In the case of Sqt1, we were able to decipher the mode of L10-N peptide binding by X-ray crystallography. These structural analyses showed that the C-terminal domain of Sqt1, which is preceded by a non-essential N-terminal extension of ∼50 amino acids, folds into an eight-bladed WD-repeat β-propeller. Moreover, the binding mode of the N-terminal residues of Rpl10 (L10-N) by the eight-bladed WD-repeat β-propeller of Sqt1, as revealed by X-ray crystallography, allows establishing a refined model for the final pre-60S maturation events that lead to the stable incorporation of Rpl10 and the release of Nmd3. Taken together, we propose that Sqt1 may protect Rpl10 from aggregation before and/or promote its incorporation into almost mature pre-60S subunits in the cytoplasm. We conclude that the β-propeller domains of Sqt1 and Rrb1, which harbour the essential function of these proteins, recognize the very N-terminal residues of Rpl10 and Rpl3.

To this end, we also performed in vitro binding assays with the orthologous proteins from the thermophilic, filamentous ascomycete Chaetomium thermophilum (ct), whose proteins often exhibit improved biochemical properties. Both ctSqt1 and ctSqt1.52C (deletion of amino acids 2–51), which fully complement the absence of Sqt1 in vivo, could be efficiently co-purified with ctRpl10 or its N-terminal 20 residues. As a first step towards the elucidation of the recognition mode of the N-terminal residues of Rpl10 by the predicted β-propeller domain of Sqt1 at the atomic level, we independently determined the crystal structure of ctSqt1 at 1.94 Å by molecular replacement and of ctSqt1.52C, lacking the dispensable N-terminal extension, at 1.5 Å resolution by single-anomalous dispersion (SAD) followed by molecular replacement using the ctSqt1.52C Se-Met structure as the search model. While the N-terminal extension could not be resolved, the crystal structures revealed that residues 52–533 of ctSqt1 form a typical eight-bladed WD-repeat β-propeller; thus, being composed of eight blades that each contain four β-strands and showing the characteristic ‘velcro' closure owing to the presence of the N-terminal β-strand as the outermost β-strand of the eighth blade. Sqt1 and ctSqt1 share a high degree of overall structural conservation and mainly differ in three ctSqt1-specific insertions located in the loops connecting β-strands 1c-1d, 5c-5d and 7c-7d. Analysis of the electrostatic properties revealed that both β-propeller structures notably contain a negatively charged top surface, whereas the bottom sides exhibit a charge-mixed surface.

> MALENDSIAYFDGHKDSVFAIAQHPLYPNIVATGGSEGDADDAPGKGYVLDISAAAGRPVLPPSYNSDPSSAPQQNTSLNPIFEIDGHTDSINALTFTLPRGDFLVSGGMDGRMRVYAVSVPQNGALAQFKFLAESQETEEINWFAPCPSPDHPNTIALGASDGSVWVFTLDASDPSNPVQIVQSYFLHTGPCTAGAWSPDGLLLATVSEDESLHVYDVFGVAASKSLVTDNGQTVVSLTNVDQRFAVEGGLFSVAVSPTGAVVAVGGAGGQIKIVGLPRLSQPQQPQSQSQSRTGKAPAGRAGRPSQQQQTTSHQAGTILASLQIQSDNIESLAFSPSAPILAAGSTDGSIAVFDTSRSFALRRHLRGAHAEDPVVKVEFVKSPPNAAMAGWLLTSCGMDGVVRRWDLRGGTAGPGTLPHMQHLQQQRQQQQEGAAPSGLVKEWKGHRSGQEGGGVLGFVQGETGERIVTVGDDAVVLVFEAGSHHHHHH> AGMSLTQVSGPVYVVEDNYYVQENSMVYFGAKGVTVVGATWTPDTARELHKLIKRVSRKPVLEVINTNYHTDRAGGNAYWKSIGAKVVSTRQTRDLMKSDWAEIV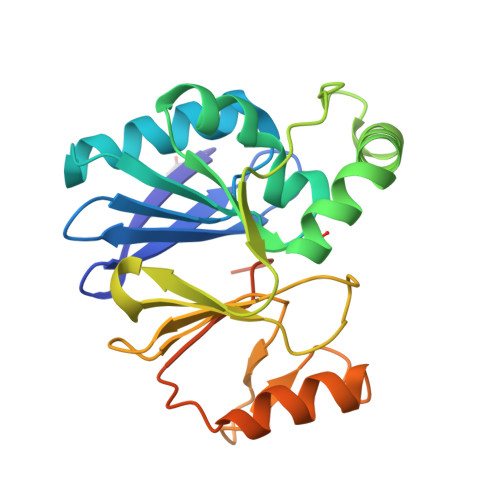AFTRKGLPEYPDLPLVLPNVVHDGDFTLQEGKVRAFYAGPAHTPDGIFVYFPDEQVLYGNDILKEKLGNLSFADVKAYPQTLERLKAMKLPIKTVIGGHDSPLHGPELIDHYEALIKAAPQS> MADQAFVTLTTNDAYAKGALVLGSSLKQHRTTRRLVVLATPQVSDSMRKVLETVFDEVIMVDVLDSGDSAHLTLMKRPELGVTLTKLHCWSLTQYSKCVFMDADTLVLANIDDLFDREELSAAPDPGWPDCFNSGVFVYQPSVETYNQLLHLASEQGSFDGGDQGILNTFFSSWAT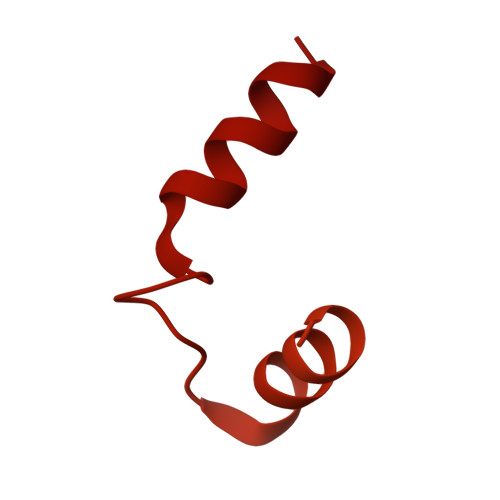TDIRKHLPFIYNLSSISIFSYLPAFKVFGASAKVVHFLGRVKPWNYTYDPKTKSVKSEAHDPNMTHPEFLILWWNIFTTNVLPLLQQFGLVKDTCSYVNVEDVSGAISHLSLGEIPAMAQPFVSSEERKERWEQGQADYMGADSFDNIKRKLDTYLQ>[4x]EDGSDPPSGDFLTEGGGVRGPRLVERQQSACKETGWPFCSDEDWNTKCPSGCRMKGLIDEVDQDFTSRINKLRDSLFNYQKNSKDSNTLTKNIVELMRGDFAKANNNDNTFKQINEDLRSRIEILRRKVIEQVQRINLLQKNVRDQLVDMKRLEVDIDIKIRSCKGSCSRALEHKVDLEDYKNQQKQLEQVIAINLLPSRDIQYLPILKMSTITGPVPREFKSQLQEAPLEWKALLEMQQTKMVLETFGGDGHARGDSVSQGTGLAPGSPRKPGTSSIGNVNPGSYGPGSSGTWNPGRPEPGSAGTWNPGRPEPGSAGTWNPGRPEPGSAGTWNPGRPEPGSAGTWNPGRPEPGSAGTWNTGSSGSSSFRPDSSGHGNIRPSSPDWGTFR;>[4x]KVERKPPDADGCLHADPDLGVLCPTGCKLQDTLVRQERPIRKSIEDLRNTVDSVSRTSSSTFQYITLLKNMWKGRQNQVQDNENVVNEYSSHLEKHQLYIDETVKNNIPTKLRVLRSILENLRSKIQKLESDVSTQMEYCRTPCTVTCNIPVVSGKECEKIIRNEGETSEMYLIQPEDSSKPYRVYCDMKTEKGGWTVIQNRQDGSVDFGRKWDPYKQGFGNIATNAEGKKYCGVPGEYWLGNDRISQLTNMGPTKLLIEMEDWKGDKVTALYEGFTVQNEANKYQLSVSKYKGTAGNALIEGASQLVGENRTMTIHNSMFFSTYDRDNDGWKTTDPRKQCSKEDGGGWWYNRCHAANPNGRYYWGGAYTWDMAKHGTDDGVVWMNWQGSWYSMKKMSKMIRPYFPEQ;>[4x]YVATRDNCCILDERFGSYCPTTCGIADFLNNYQTSVDKDLRTLEGILYQVENKTSEARELVKAIQISYNPDQPSKPNNIESATKNSKSMMEEIMKYETLISTHESTIRFLQEIYNSNSQKIVNLRDKVVQLE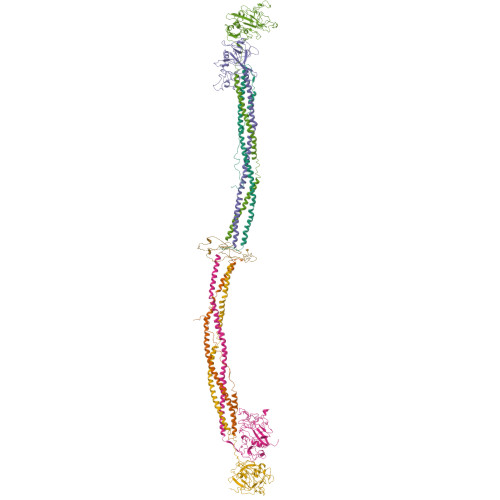ANCQEPCQDTVKIHDVTGRDCQDVANKGAKESGLYFIRPLKAKQQFLVYCEIDGSGNGWTVFQKRLDGSLDFKKNWIQYKEGFGHLSPTGNTEFWLGNEKIHLISTQSTIPYVLRIQLEDWNGRTSTADYASFKVTGENDKYRLTYAYFIGGDAGDAFDGYDFGDDSSDKFFTSHNGMQFSTWDSDNDKYDGNCAEQDGSGWWMNKCHAGHLNGVYYQGGTYSKTSTPNGYDNGIIWATWKSRWYSMKKTTMKIIPLNRLAIGEGQQHQLGGAKQAGDV> AGNFWQSSHYLQWILDKQDLLKERQKDLKFLSEEEYWKLQIFFTNVIQALGEHLKLRQQVIATATVYFKRFYARYSLKSIDPVLMAPTCVFLASKVEEFGVVSNTRLIAAATSVLKTRFSYAFPKEFPYRMNHILECEFYLLELMDCCLIVYHPY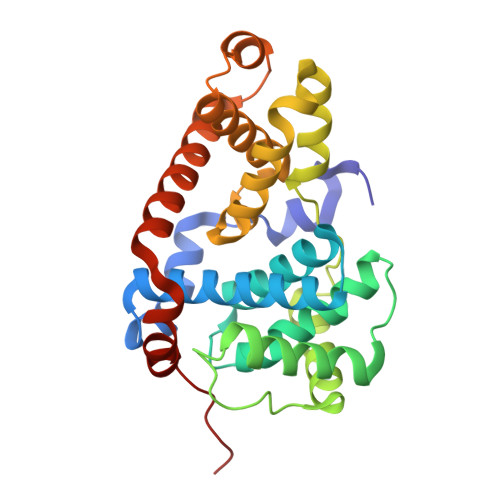RPLLQYVQDMGQEDMLLPLAWRIVNDTYRTDLCLLYPPFMIALACLHVACVVQQKDARQWFAELSVDMEKILEIIRVILKLYEQWKNFDERKEMATILSKMPKPKPPP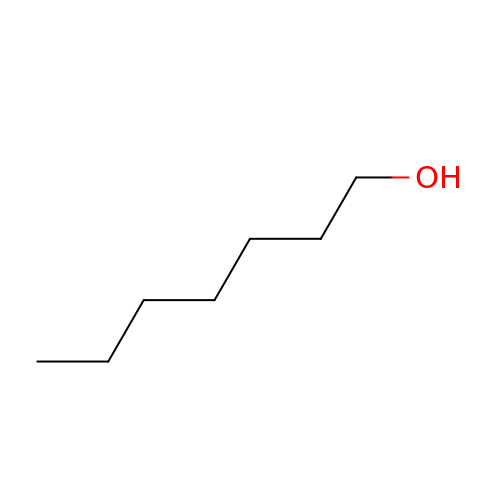HEPTAN-1-OL | C7 H16 O | BBMCTIGTTCKYKF-UHFFFAOYSA-N> GKLSLQDVAELIRARACQRVVVMVGAGISTPSGIPDFRSPGS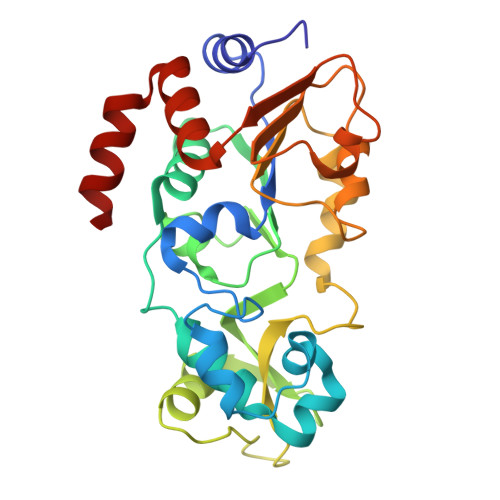GLYSNLQQYDLPYPEAIFELPFFFHNPKPFFTLAKELYPGNYKPNVTHYFLRLLHDKGLLLRLYTQNIDGLERVSGIPASKLVEAHGTFASATCTVCQRPFPGEDIRADVMADRVPRCPVCTGVVKPDIVFFGEPLPQRFLLHVVDFPMADLLLILGTSLEVEPFASLTEAVRSSVPRLLINRDLVGPLAWHPRSRDVAQLGDVVHGVESLVELLGWTEEMRDLVQRET>MRHDGRQHDELRPITFDLDFISHPEGSVLITAGNTKVICNASVEDRVPPFLRGGGKGWITAEYSMLPRATNQRTIRESSKGKISGRTMEIQRLIGRALRAVVDLEKLGERTIWIDCDVIQADGGTRTASITGAFLAMAIAIGKLIKAGTIKTNPITDFL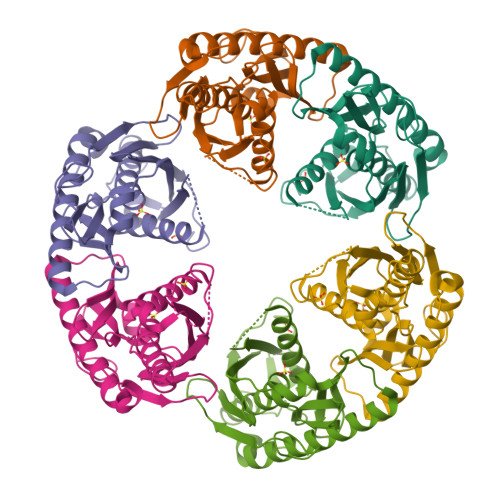AAISVGIDKEQGILLDLNYEEDSSAEVDMNVIMTGSGRFVELQGTGEEATFSREDLNGLLGLAEKGIQELIDKQKEVLGDSLPELK[6x]(2S)-1-[(13-bromotridecanoyl)oxy]-3-hydroxypropan-2-yl 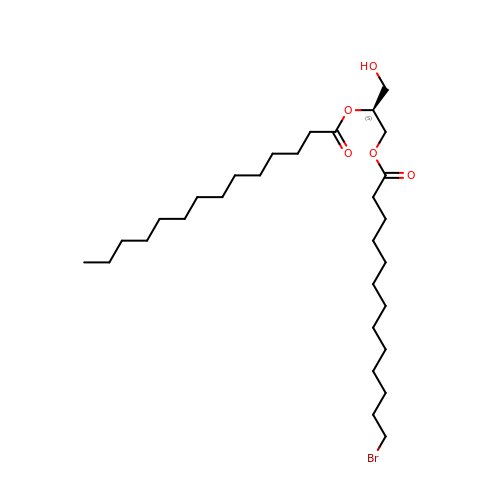tetradecanoate | C30 H57 Br O5 | VHCCBJMTBOAHLF-NDEPHWFRSA-N>GVSGHRDMISTRRLPPSIVQDTILAVVPPKSCAAIGTDVDLRDWGFDTFEVASRVPSVLQSVAMHVALAWDFFASQEEAQKWAFLVAAVENNYRPNPYHNAIHAADVLQGTFSLVSAAKPLMEHLTPLECKAAAFAALTHDVCHPGRTNAFLAAVQDPVSFKFSGKGTLEQLHTATAFELLNVTEFDFTSSMDNASFLEFKNIVSHLIGHTDMSLHSETVAKHGAKLSAGGFDCTCKEDRLEALSLLLHAADIGASSRGVAIARKWLVILQEFADQAEDERRRGLPVTPGFETPSSVEKSQIPFLDFFVIPTFDLLHQLFPSIEEPLHNLRKLRELYAAKAGV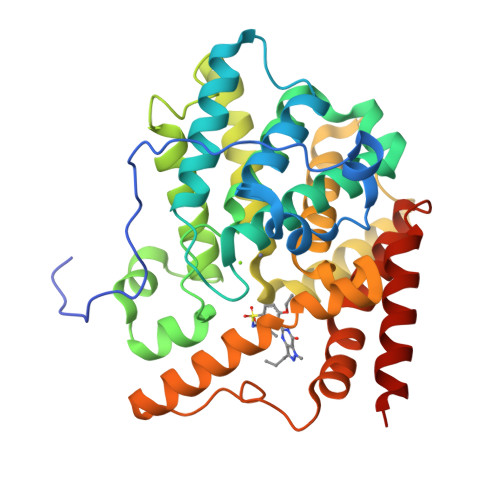TT[8x]>PNFSGNWKIIRSENFEELLKVLGVNVMLRKIAVAAASKPAVEIKQEGDTFYIKVSTTVR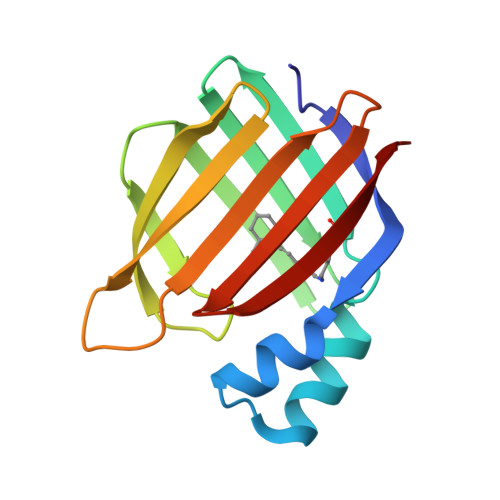TTEINFKVGEEFEEQTVDGRPCKSLVKWESENKMVCEQKLLKGEGPKTSWTLELTNDGELIDTMTADDVVCTKVFVRE[2x]The exo-β-1,3-galactanase is a glycoside hydrolase from the basidiomycete Phanerochaete chrysosporium (Pc1,3Gal43A), which specifically cleaves AGPs. In this context, exo-β-1,3-galactanase (EC 3.2.1.145) specifically cleaves the nonreducing end β-1,3–linked galactosyl linkage of β-1,3-galactans to release d-galactose (Gal). In this study, we solved the apo and liganded structures of Pc1,3Gal43A, which reveal a glycoside hydrolase family 43 subfamily 24 (GH43_sub24) catalytic domain together with a carbohydrate-binding module family 35 (CBM35) binding domain. The N-terminal catalytic domain consists of a five-bladed β-propeller (Gln21–Gly325), as in other GH clan-F enzymes, and the C-terminal domain (PcCBM35) takes a β-jellyroll fold (Thr326–Tyr448) structure, as in previously reported CBM35s.

The crystal structure of the SeMet derivative of Pc1,3Gal43A was first determined by means of the multiwavelength anomalous dispersion method, and this was followed by structure determination of the ligand-free WT, the WT bound with Gal (WT_Gal), the E208Q mutant co-crystallized with β-1,3-galactotriose (Gal3; E208Q_Gal3), and the E208A mutant co-crystallized with Gal3 (E208A_Gal3). No Gal3 molecule was observed at the catalytic domain in the structure of the Gal3 co-crystallized E208A mutant. In E208A_Gal3, electron density of Gal3 was observed in the ligand-binding site of PcCBM35. 2Fo − Fc omit maps showed that the binding mode of PcCBM35 with ligands is “exo-type,” corresponding to type-C CBM. The asymmetric unit of E208A_Gal3 contained four Pc1,3Gal43A molecules, and each molecule binds to the nonreducing end of Gal3 (called Gal_site 1), as in other CBM35 modules. However, the middle Gal (Gal_site 2) and the reducing end Gal (Gal_site 3) are found in two main locations, although residues involved in the interactions with the ligand in each molecule were mostly shared. The Gal_site 1 forms hydrogen bonds with Tyr355 and Arg388 and interacts hydrophobically with Leu342, Gly354, Tyr438, and Asp441. The Gal_site 2 interacts hydrophobically with Gly383 and Asp384. However, ensemble refinement revealed that Gal_site 1 and Gal_site 2 do not show huge fluctuations, whereas Gal_site 3 has many conformations. At the catalytic site, Gal−1 is anchored in the appropriate position, and Gal+2 appears to fluctuate in a planar fashion as it interacts with the surrounding residues. In the CBM, it was inferred that Gal_site 1 is fixed and Gal_site 3 is adsorbed at the appropriate location at the binding site while fluctuating in three dimensions.

>NQIVSGAAWTDTAGNTIQAHGAGILQVGSTFYWFGEDKSHNSALFKAVSCYTSSDLVNWSRQNDALSPIAGTMISTSNVVERPKVIFNQKNSEYVMWFHSDSSNYGAAMVGVATAKTPCGPYTYKGSFKPLGADSRDESIFQDDDSAQTAYLLYASDNNQNFKISRLDANYYNVTAQVSVMNGATLAAPGIVKHNGEYFLIASHTSGWAPNPNKWFSASSLAGPWSAQQDIAPSATRTWYSQNAFDLPLGSNAIYMGDRWRPSLLGSSRYIWYPLDFSSGAPQIVHADVWSVNVQAGTYSVASGTSYEAENGQRGGSSTILSGSGFSGGKAVGYLGHGGTVTINNVQSNGGSHWVALYFANGDSTYRNVTVSVNGGPSVLVDQPDSGGGNVVISVPVKLNLNSGENSITFGSGQSNYAADLDKIIVY[4x]>SNAMDKIVVQGGDNRLVGSVTIEGAKNAVLPLLAATILASEGKTVLQNVPILSDVFIMNQVVGGLNAKVDFDEEAHLVKVDATGDITEEAPYKYVSKMRASIVVLGPILARVGHAKVSMPGGCTIGSRPIDLHLKGLEAMGVKISQTAGYIEAKAERLHGAHIYMDFP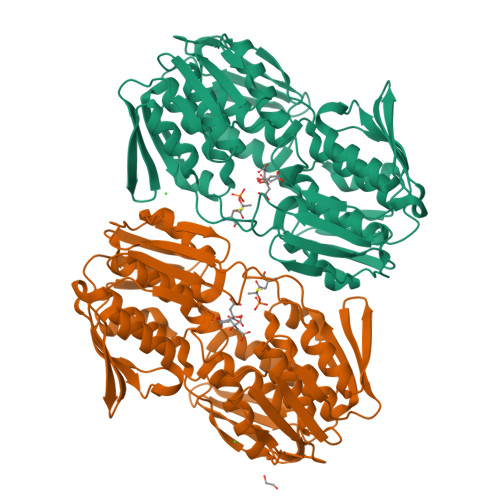SVGATQNLMMAATLADGVTVIENAAREPEIVDLAILLNEMGAKVKGAGTETITITGVEKLHGTTHNVVQDRIEAGTFMVAAAMTGGDVLIRDAVWEHNRPLIAKLLEMGVEVIEEDEGIRVRSQLENLKAVHVKTLPHPGFPTDMQAQFTALMTVAKGESTMVETVFENRFQHLEEMRRMGLHSEIIRDTARIVGGQPLQGAEVLSTDLRASAALILTGLVAQGETVVGKLVHLDRGYYGFHEKLAQLGAKIQRIEASDEDE[2x]> MKLDIKKTFSNRSDRVKGIDFHPTEPWVLTTLYSGRVEIWNYETQVEVRSIQVTETPVRAGKFIARKNWIIVGSDDFRIRVFNYNTGEKVVDFEAHPDYIRSIAVHPTKPYVLSGSDDLTVKLWNWENNW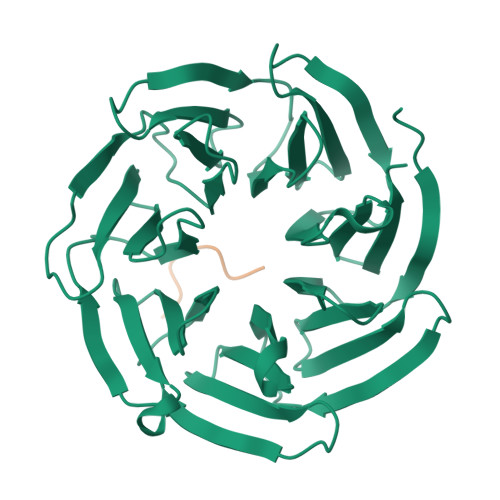ALEQTFEGHEHFVMCVAFNPKDPSTFASGCLDRTVKVWSLGQSTPNFTLTTGQERGVNYVDYYPLPDKPYMITASDDLTIKIWDYQTKSCVATLEGHMSNVSFAVFHPTLPIIISGSEDGTLKIWNSSTYKVEKTLNVGLERSWCIATHPTGRKNYIASGFDNGFTVLSLG;> ELVIKTSHDD4-(1-methyl-1-phenylethyl)phenol | C15 H16 O | 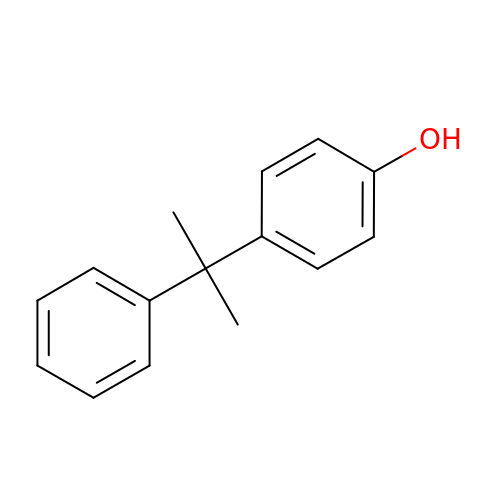QBDSZLJBMIMQRS-UHFFFAOYSA-N>[2x]MRRLEEDAVRVAYAGLRRKEAFKALAEKLGFTPLLFPVQATEKVPVPEYRDQVRALAQGVDLFLATTGVGVRDLLEAGKALGLDLEGPLAKAFRLARGAKAARALKEAGLPPHAVGDGTSKSLLPLLPQGRGVAALQLYGKPLPLLENALAERGYRVLPLMPYRHLPDPEGILRLEEALLRGEVDALAFVAAIQVEFLFEGAKDPKALREALNTRVKALAVGRVTA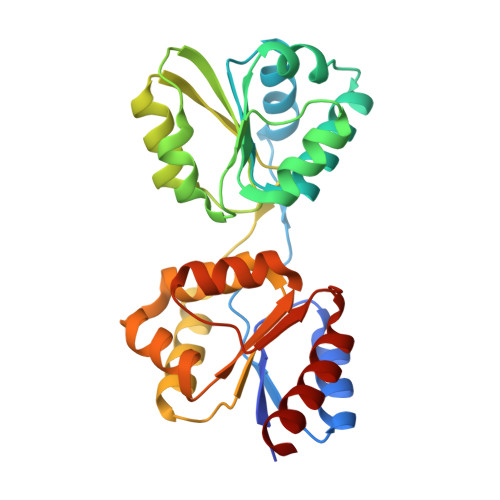DALREWGVKPFYVDETERLGSLLQGFKRALQKEVA> GGUUGCCGAAUCCAUGUCGUUUGGUACGGAGGAACCGCUUUUUGGGGUUAAUCUGCAGUGAAGCUGCAGUAGGGAUACCUUCUGUCCCGCACCCGACAGCUAACUCCGGA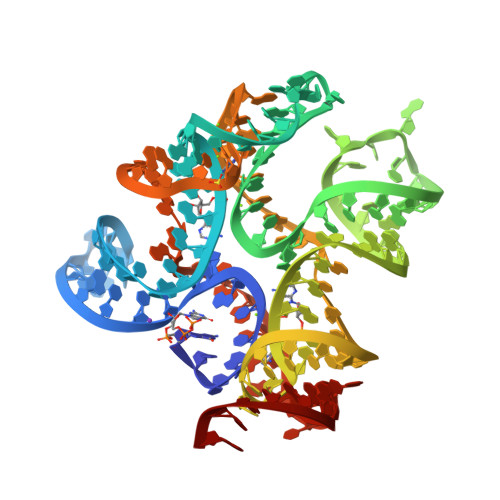GGCAAUAAAGGAAGGAG> MLQDADRTRILAISPHLDDAVLSVGASLAQAEQDGGKVTVFTVFAGSAAPPYSPAAERFHARWGLSPTEDAPLRRRNEDIAALDQLGAGHRHGRF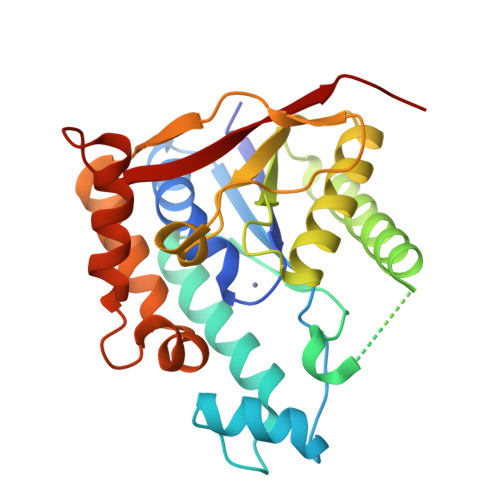LDAIYRRSPDGQWLLHHNEGSMVRQQSPANNHDLVAAIREDIESMIAECDPTLVLTCVAIGKHPDHKATRDATLLAARERGIPLRLWQDLPYAAYSQDLAELPDGLRLGSPELSFVDEEARTRKFQAMKHYATQLSVLDGPNKNLFAKLDEHARNAAPDGGYNETTWPVIRYAAE>[4x]MLEIKRYKNRVASRKSRAKFK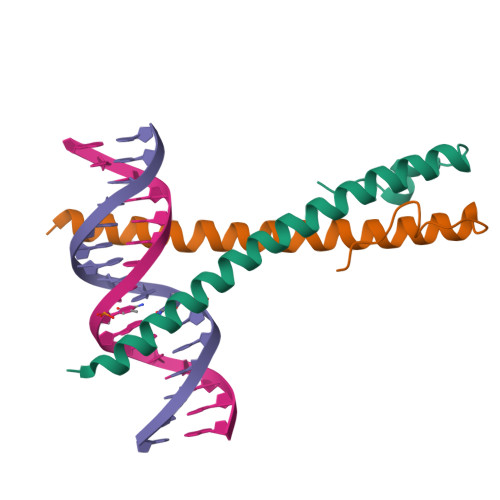QLLQHYREVAAAKSSENDRLRLLLKQMCPSLDVDSIIPRTPD>MFEARLVQGSILKKVLEALKDLINEACWDISSSGVNLQSMDSSHVSLVQLTLRSEGFDTYRCDRNLAMGVNLTSMSKILKCAGNEDIITLRAEDNADTLALVFEAPNQEKVSDYEMKLMDLDVEQLGIPEQEYSCVVKMPSGEFARICR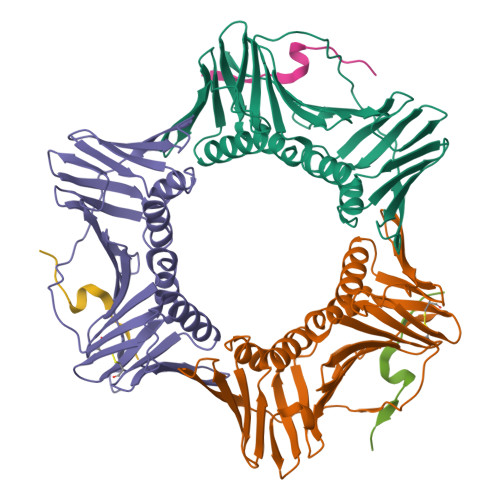DLSHIGDAVVISCAKDGVKFSASGELGNGNIKLSQTSNVDKEEEAVTIEMNEPVQLTFALRYLNFFTKATPLSSTVTLSMSADVPLVVEYKIADMGHLKYYLAPKIEDEE[3x];>[3x]KRRQTSMTDFYHSKR> YGTQIAEITAREILDSRGRPTVEAEVHLEDGSVGLAQVPSGASTGTFEAHELRDDDPSRYGGKGVQKAVENVSAIEDALIGLSALDQEGLDKAMIALDGTPNKKNLGANAILAVSLATAHAAATSLNLPLYRYLGGPLANVLPVPMMNVINGGAHADNNVDFQEFMIMPVGAPSFKEALRWGAEVFHALAK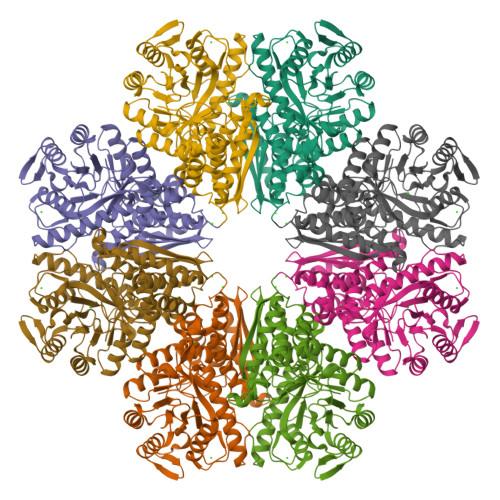VLKDKGLATGVGDEGGFAPNLGSNKEALELLLTAIEAAGYKPGEQVALAMDVASSEFYKNGLYTCDGVSHEPAGMIGILADLVSQYPIVSIEDGLQEDDWSNWKTLTQQLGSTVQLVGDDLFVTNPDRLQSGIEQGVGNAVLIKLNQIGTLTETLRTIDLATRSGYRSVISHRSGETEDTTIADLAVATRAGQIKTGSLSRSERIAKYNRLLRIEAALGENALYAGAIGLGPK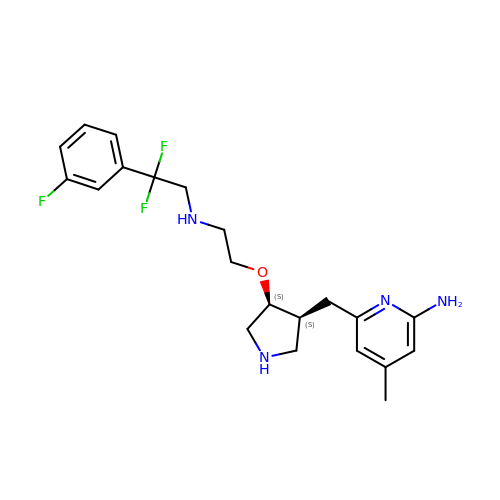6-{[(3S,4S)-4-(2-{[2,2-difluoro-2-(3-fluorophenyl)ethyl]amino}ethoxy)pyrrolidin-3-yl]methyl}-4-methylpyridin-2-amine | C21 H27 F3 N4 O | IRAITVAESBBILD-HNAYVOBHSA-N> MHHHHHHMIEWIIRRSVANRFLVLMGALFLSIWGTWTIINTPVDALPDLSDVQVIIKTSYPGQAPQIVENQVTYPLTTTMLSVPGAKTVRGFSQFGDSYVYVIFEDGTDPYWARSRVLEYLNQVQGKLPAGVSAELGPDATGVGWIYEYALVDRSGKHDLADLRSLQDWFLKYELKTIPDVAEVASVGGVVKEYQVVIDPQRLAQYGISLAEVKSALDASNQEAGGSSIELAEAEYMVRASGYLQTLDDFNHIVLKASENGVPVYLRDVAKVQIGPEMRRGIAELNGEGEVAGGVVILRSGKNAREVIAAVKDKLETLKSSLPEGVEIVTTYDRSQLIDRAIDNLSGKLLEEFIVVAVVCALFLWHVRSALVAIISLPLGLCIAFIVMHFQGLNANIMSLGGIAIAVGAMVDAAIVMIENAHKRLEEWQHQHPDATLDNKTRWQVITDASVEVGPALFISLLIITLSFIPIFTLEGQEGRLFGPLAFTKTYAMAGAALLAIVVIPILMGYWIRGKIPPESSNPLNRFLIRVYHPLLLKVLHWPKTTLLVAALSVLTVLWPLNKVGGEFLPQINEGDLLYMPSTLPGISAAEAASMLQKTDKLIMSVPEVARVFGKTGKAETATDSAPLEMVETTIQLKPQEQWRPGMTMDKIIEELDNTVRLPGLANLWVPPIRNRIDMLSTGIKSPIGIKVSGTVLADIDAMAEQIEEVARTVPGVASALAFRLEGGRYINVEINREKAARYGMTVADVQLFVTSAVGGAMVGETVEGIARYPINLRYPQSWRDSPQALRQLPILTPMKQQITLADVADIKVSTGPSMLKTENARPTSWIYIDARDRDMVSVVHDLQKAIAEKVQLKPGTSVAFSGQFELLERANHKLKLMVPMTLMIIFVLLYLAFRRVGEALLIISSVPFALVGGIWLLWWMGFHLSVATGTGFIALAGVAAEFGVVMLMYLRHAIEAVPSLNNPQTFSEQKLDEALYHGAVLRVRPKAMTVAVIIAGLLPILWGTGAGSEVMSRIAAPMIGGMITAPLLSLFIIPAAYKLM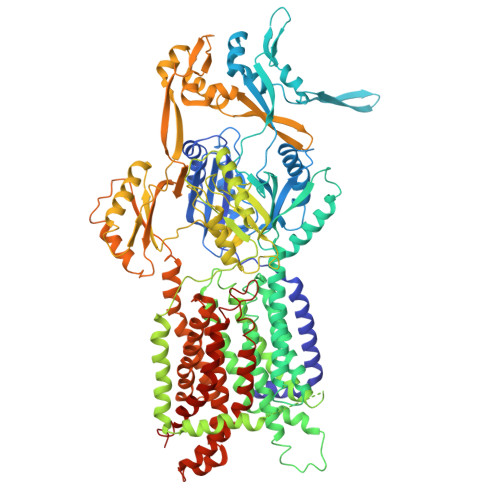WLHRHRVRK>MEFTTGLMSLDTALNEMLSRVTPLTAQETLPLVQCFGRILASDVVSPLDVPGFDNSAMDGYAVRLADIASGQPLPVAGKSFAGQPYHGEWPAGTCIRIMTGAPVPEGCEAVVMQEQTEQMDNGVRFTAEVRSGQNIRRRGEDISAGAVVFPAGTRLTTAELPVIASLGIAEVPVIRKVRVALFSTGDALQLPGQPLGDGQIYDTNRLAVHLMLEQLGCEVINLGIIRDDPHALRAAFIEADSQADVVISSGGVSVGEADYTKTILEELGEIAFWKLAIK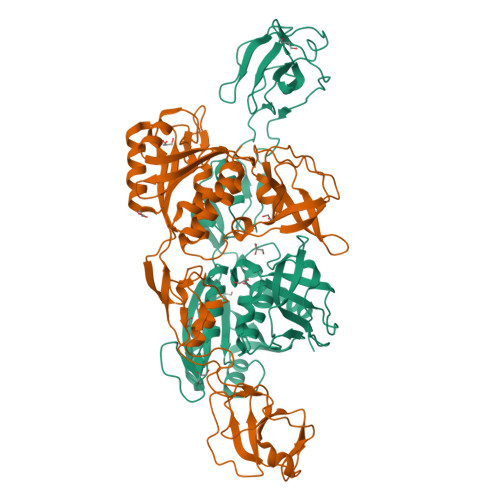PGKPFAFGKLSNSWFCGLPGNPVSATLTFYQLVQPLLAKLSGNTASGLPARQRVRTASRLKKTPGRLDFQRGVLQRNADGELEVTTTGHQGSHIFSSFSLGNCFIVLERDRGNVEVGEWVEVEPFNALFGGL[2x]>[3x]PIELLPETPSQTAGPYVHIGLALEAAGNPTRDQEIWNRLAKPDAPGEHILLLGQVYDGNGHLVRDSFLEVWQADANGEYQDAYNLENAFNSFGRTATTFDAGEWTLHTVKPGVVNNAAGVPMAPHINISLFARGINIHLHTR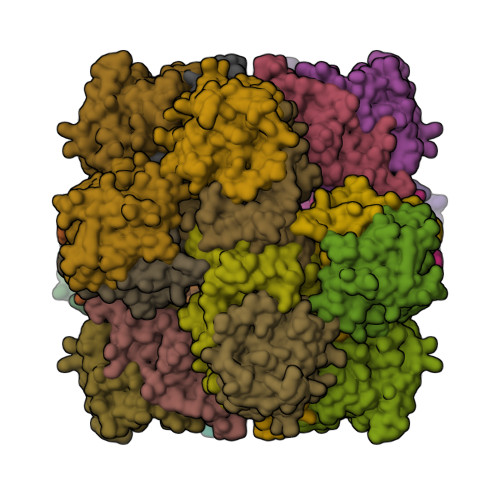LYFDDEAQANAKCPVLNLIEQPQRRETLIAKRCEVDGKTAYRFDIRIQGEGETVFFDF;>PAQDNSRFVIRDRNWHPKALTPDYKTSIARSPRQALVSIPQSISETTGPNFSHLGFGAHDHDLLLNFNNGGLPIGERIIVAGRVVDQYGKPVPNTLVEMWQANAGGRYRHKNDRYLAPLDPNFGGVGRCLTDSDGYYSFRTIKPGPHPWRNGPNDWRPAHIHFGISGPSIATKLITQLYFEGDPLIPMCPIVKSIANPEAVQQLIAKLDMNNANPMDCLAYRFDIVLRGQRKTHFENC[3x]> MPETFEAIARAIEVAREVEKVAQRAEEEGN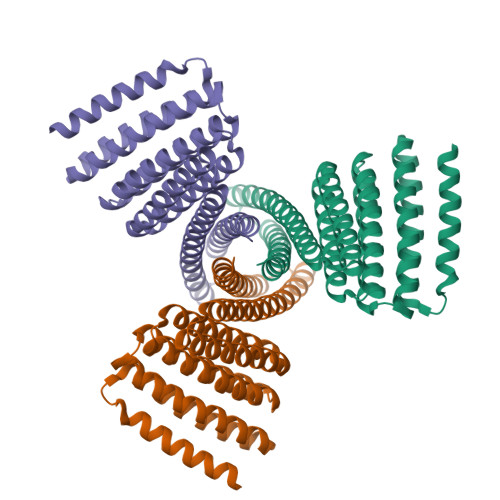PDLRDSAKELARAVDEAIEEAKKQGNPELVEWVARAAKVAAEVIKVAIQAEKEGNRDLFRAALELVRAVIEAIEEAVKQGNPELVEWVARAAKVAAEVIKVAIQAEKEGARDLFRLALELVRAVIEAIEFAVKLGDPEMVERAARIAKTAAELIKRAIRAKKEGDKDQEREAKKRVTRLIIELTLMVLKASLDLLRRILEELKEMLERLEKNPDKDVIVKVLKVIVKAIEASVDNQRVSADNQKMLAELAGSWSGGGSEQKLISEEDLGGS>[4x]GPGDPP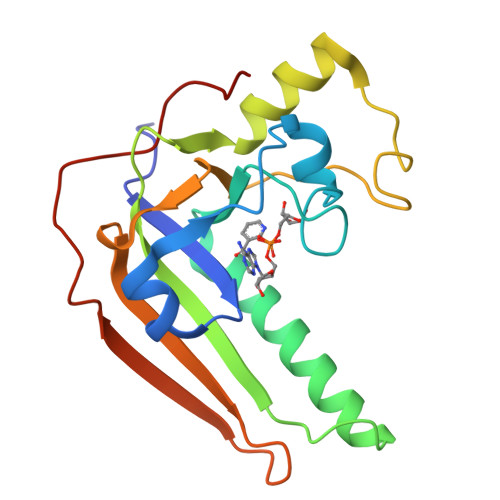ATVYRYDSRPPEDVFQNGFTAWGNNDNVLEHLTGRSSQVGSSNSAFVSTSSSRRYTEVYLEHRMQEAVEAERAGRGTGHFIGYIYEVRADNNFYGAASSYFEYVDTYGDNAGRILAGALATYQSEYLAHRRIPPENIRRVTRVYHNGITGETTTTEYSNARYVSQQTRANPNPYTSRR Human 5′‐3′ exonuclease PLD3, a member of the phospholipase D family of enzymes, has been validated as a therapeutic target for treating Alzheimer's disease. We could not measure any phospholipase activity but the enzyme shows robust nuclease activity.

Here, we have determined the crystal structure of the luminal domain of the enzyme at 2.3 Å resolution, revealing a bilobal structure with a catalytic site located between the lobes. We then compared the structure with published crystal structures of other human PLD family members which revealed that a number of catalytic and lipid recognition residues, previously shown to be key for phospholipase activity, are not conserved or, are absent. This led us to test whether the enzyme is actually a phospholipase. Finally, we have mapped key single nucleotide polymorphisms onto the structure which reveals plausible reasons as to why they have an impact on Alzheimer's disease.

>MKPKLMYQELKVPAEEPANELPMNEIEAWKAAEKKARWVLLVLILAVVGFGALMTQLFLWEYGDLHLFGPNQRPAPCYDPCEAVLVESIPEGLDFPNASTGNPSTSQAWLGLLAGAHSSLDIASFYWTLTNNDTHTQEPSAQQGEEVLRQLQTLAPKGVNVRIAVSKPSGPQPQADLQALLQSGAQVRMVDMQKLTHGVLHTKFWVVDQTHFYLGSANMDWRSLTQVKELGVVMYNCSCLARDLTKIFEAYWFLGQAGSSIPSTWPRFYDTRYNQETPMEICLNGTPALAYLASAPPPLCPSGRTPDLKALLNVVDNARSFIYVAVMNYLPTLEFSHPHRFWPAIDDGLRRATYERGVKVRLLISCWGHSEPSMRAFLLSLAALRDNHTHSDIQVKLFVVPADEAQARIPYARVNHNKYMVTERATYIGTSNWSGNYFTETAGTSLLVTQNGRGGLRSQLEAIFLRDWDSPYSHDLDTSADSVGNACRLL[2x]> SNAMAKTLKDLQGWEIITTDEQGNIIDGGQKRLRRRGAKTEHYLKRSSDGIKLGRGDSVVMHNEAAGTYSVYMIQELRLNTLNNVVELWALTYLRWFEVNPLAHYRQFNPDANILNRPLNYYNKLFSETANKNELYLTAELAELQLFNFIRVANVMDGSKWEVLKGNVDPERDFTVRYICEPTGEKFVDINIEDVKAYIKKVEPREAQEYLKDLTLPSKKKEIKRGPQKKDKATQTAQISDAETRATDITDNEDGNEDESSDYESPSDIDVSEDMDSGEISADELEEEEDEEEDEDEEEKEARHTNSPRKRGRKIKLGKDDIDASVQPPPKKRGRKPKDPSKPRQMLLISSCRANNTPVIRKFTKKNVARAKKKYTPFSKRFKSIAAIPDLTSLPEFYGNSSELMASRFENKLKTTQKHQIVETIFSKVKKQLNSSYVKEEILKSANFQDYLPARENEFASIYLSAYSAIESDSATTIYVAGTPGVGKTLTVREVVKELLSSSAQREIPDFLYVEINGLKMVKPTDCYETLWNKVSGERLTWAASMESLEFYFKRVPKNKKKTIVVLLDELDAMVTKSQDIMYNFFNWTTYENAKLIVIAVANTMDLPERQLGNKITSRIGFTRIMFTGYTHEELKNIIDLRLKGLNDSFFYVDTKTGNAILIDAAGNDTTVKQTLPEDVRKVRLRMSADAIEIASRKVASVSGDARRALKVCKRAAEIAEKHYMAKHGYGYDGKTVIEDENEEQIYDDEDKDLIESNKAKDDNDDDDDNDGVQTVHITHVMKALNETLNSHVITFMTRLSFTAKLFIYALLNLMKKNGSQEQELGDIVDEIKLLIEVNGSNKFVMEIAKTLFQQGSDNISEQLRIISWDFVLNQLLDAGILFKQTMKNDRICCVKLNISVEEAKRAMNEDETLRNL;> MLNGEDFVEHNDILSSPAKSRNVTPKRVDPHGERQLRRIHSSKKNLLERISLVGNERKNTSPDPALKPKTPSKAPRKRGRPRKIQEELTDRIKKDEKDTISSKKKRKLDKDTSGNVNEESKTSNNKQVMEKTGIKEKREREKIQVATTTYEDNVTPQTDDNFVSNSPEPPEPATPSKKSLTTNHDFTSPLKQIIMNNLKEYKDSTSPGKLTLSRNFTPTPVPKNKKLYQTSETKSASSFLDTFEGYFDQRKIVRTNAKSRHTMSMAPDVTREEFSLVSNFFNENFQKRPRQKLFEIQKKMFPQYWFELTQGFSLLFYGVGSKRNFLEEFAIDYLSPKIAYSQLAYENELQQNKPVNSIPCLILNGYNPSCNYRDVFKEITDLLVPAELTRSETKYWGNHVILQIQKMIDFYKNQPLDIKLILVVHNLDGPSIRKNTFQTMLSFLSVIRQIAIVASTDHIYAPLLWDNMKAQNYNFVFHDISNFEPSTVESTFQDVMKMGKSDTSSGAEGAKYVLQSLTVNSKKMYKLLIETQMQNMGNLSANTGPKRGTQRTGVELKLFNHLCAADFIASNEIALRSMLREFIEHKMANITKNNSGMEIIWVPYTYAELEKLLKTVLNTL;> MSDLNQSKKMNVSEFADAQRSHYTVYPSLPQSNKNDKHIPFVKLLSGKESEVNVEKRWELYHQLHSHFHDQVDHIIDNIEADLKAEISDLLYSETTQKRRCFNTIFLLGSDSTTKIELKDESSRYNVLIELTPKESPNVRMMLRRSMYKLYSAADAEEHPTIKYEDINDEDGDFTEQNNDVSYDLSLVENFKRLFGKDLAMVFNFKDVDSINFNTLDNFIILLKSAFKYDHVKISLIFNINTNLSNIEKNLRQSTIRLLKRNYHKLDVSSNKGFKYGNQIFQSFLDTVDGKLNLSDRFVEFILSKMANNTNHNLQLLTKMLDYSLMSYFFQNAFSVFIDPVNVDFLNDDYLKILSRCPTFMFFVEGLIKQHAPADEILSLLTNKNRGLEEFFVEFLVRENPINGHAKFVARFLEEELNITNFNLIELYHNLLIGKLDSYLDRWSACKEYKDRLHFEPIDTIFQELFTLDNRSGLLTQSIFPSYKSNIEDNLLSWEQVLPSLDKENYDTLSGDLDKIMAPVLGQLFKLYREANMTINIYDFYIAFRETLPKEEILNFIRKDPSNTKLLELAETPDAFDKVALILFMQAIFAFENMGLIKFQSTKSYDLVEKCVWRGI;> SNAMTISEARLSPQVNLLPIKRHSNEEVEETAAILKKRTIDNEKCKDSDPGFGSLQRRLLQQLYGTLPTDEKIIFTYLQDCQQEIDRIIKQSIIQKESHSVILVGPRQSYKTYLLDYELSLLQQSYKEQFITIRLNGFIHSEQTAINGIATQLEQQLQKIHGSEEKIDDTSLETISSGSLTEVFEKILLLLDSTTKTRNEDSGEVDRESITKITVVFIFDEIDTFAGPVRQTLLYNLFDMVEHSRVPVCIFGCTTKLNILEYLEKRVKSRFSQRVIYMPQIQNLDDMVDAVRNLLTVRSEISPWVSQWNETLEKELSDPRSNLNRHIRMNFETFRSLPTLKNSIIPLVATSKNFGSLCTAIKSCSFLDIYNKNQLSNNLTGRLQSLSDLELAILISAARVALRAKDGSFNFNLAYAEYEKMIKAINSRIPTVAPTTNVGTGQSTFSIDNTIKLWLKKDVKNVWENLVQLDFFTEKSAVGLRDNATAAFYASNYQFQGTMIPFD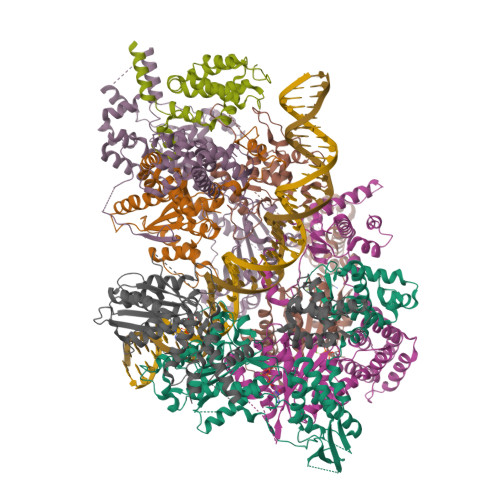LRSYQMQIILQELRRIIPKSNMYYSWTQL;> MNVTTPEVAFREYQTNCLASYISADPDITPSNLILQGYSGTGKTYTLKKYFNANPNLHAVWLEPVELVSWKPLLQAIARTVQYKLKTLYPNIPTTDYDPLQVEEPFLLVKTLHNIFVQYESLQEKTCLFLILDGFDSLQDLDAALFNKYIKLNELLPKDSKINIKFIYTMLETSFLQRYSTHCIPTVMFPRYNVDEVSTILVMSRCGELMEDSCLRKRIIEEQITDCTDDQFQNVAANFIHLIVQAFHSYTGNDIFALNDLIDFKWPKYVSRITKENIFEPLALYKSAIKLFLSTDDNLSENGQGESAITTNRDDLENSQTYDLSIISKYLLIASYICSYLEPRYDASIFSRKTRIIQGRAAYGRRKKKEVNPRYLQPSLFAIERLLAIFQAIFPIQGKAESGSLSALREESLMKANIEVFQNLSELHTLKLIATTMNKNIDYLSPKVRWKVNVPWEIIKEISESVHFNISDYFSDIHE;> MSMQQVQHCVAEVLRLDPQEKPDWSSGYLKKLTNATSILYNTSLNKVMLKQDEEVARCHICAYIASQKMNEKHMPDLCYYIDSIPLEPKKAKHLMNLFRQSLSNSSPMKQFAWTPSPKKNKRSPVKNGGRFTSSDPKELRNQLFGTPTKVRKSQNNDSFVIPELPPMQTNESPSITRRKLAFEEDEDEDEEEPGNDGLSLKSHSNKSITGTRNVDSDEYENHESDPTSEEEPLGVQESRSGRTKQNKAVGKPQSELKTAKALRKRGRIPNSLLVKKYCKMTTEEIIRLCNDFELPREVAYKIVDEYNINASRLVCPWQLVCGLVLNCTFIVFNERRRKDPRIDHFIVSKMCSLMLTSKVDDVIECVKLVKELIIGEKWFRDLQIRYDDFDGIRYDEIIFRKLGSMLQTTNILVTDDQYNIWKKRIEMDLALTEPL;> SNAMSAIPITPTKRIRRNLFDDAPATPPRPLKRKKLQFTDVTPESSPEKLQFGSQSIFLRTKALLQKSSELVNLNSSDGALPARTAEYEQVMNFLAKAISEHRSDSLYITGPPGTGKTAQLDMIIRQKFQSLPLSLSTPRSKDVLRHTNPNLQNLSWFELPDGRLESVAVTSINCISLGEPSSIFQKIFDSFQDLNGPTLQIKNMQHLQKFLEPYHKKTTFVVVLDEMDRLLHANTSETQSVRTILELFLLAKLPTVSFVLIGMANSLDMKDRFLSRLNLDRGLLPQTIVFQPYTAEQMYEIVIQKMSSLPTIIFQPMAIKFAAKKCAGNTGDLRKLFDVLRGSIEIYELEKRFLLSPTRGSLNSAQVPLTPTTSPVKKSYPEPQGKIGLNYIAKVFSKFVNNNSTRTRIAKLNIQQKLILCTIIQSLKLNSDATIDESFDHYIKAITKTDTLAPLQRNEFLEICTILETCGLVSIKKTKCKGKTKRFVDKIDVDLDMREFYDEMTKISILKPFLH>MHFTIQREALLKPLQLVAGVVERRQTLPVLSNVLLVVEGQQLSLTGTDLEVELVGRVVLEDAAEPGEITVPARKLMDICKSLPNDVLIDIRVEEQKLLVKAGRSRFTLSTLPANDFPTVEEGPGSLNFSIAQSKLRRLIDRTSFAMAQQDVRYYLNGMLLEVNGGTLR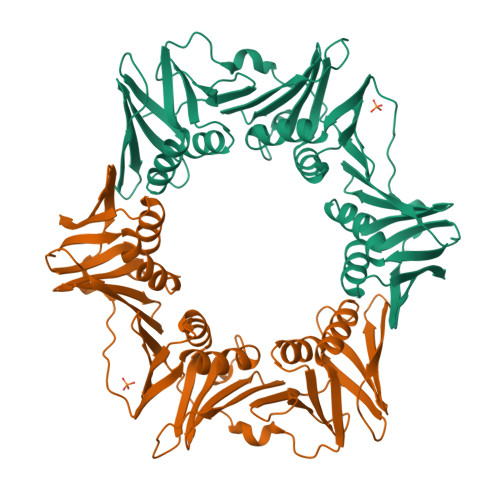SVATDGHRLAMCSLDAQIPSQDRHQVIVPRKGILELARLLTEQDGEVGIVLGQHHIRATTGEFTFTSKLVDGKFPDYERVLPRGGDKLVVGDRQQLREAFSRTAILSNEKYRGIRLQLSNGLLKIQANNPEQEEAEEEVQVEYNGGNLEIGFNVSYLLDVLGVIGTEQVRFILSDSNSSALVHEADNDDSAYVVMPMRL[4x]>[4x]GAMGQTSTRWTPTTEQIKILKELYYNNAIRSPTADQIQKITAR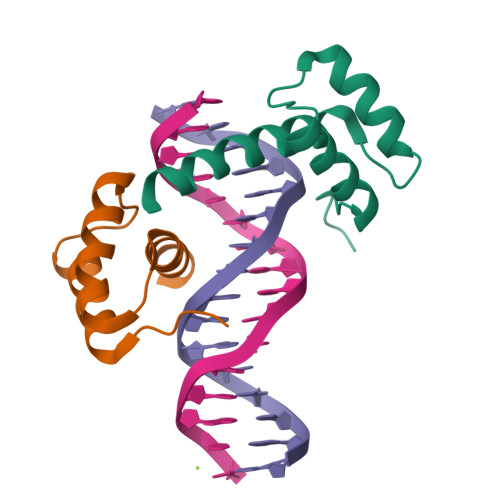LRQFGKIEGKNVFYWFQNHKARERQKKRFNGGS>[2x]HGSPVDICTAKPRDIPMNPMCIYRSPEKKATEDEGS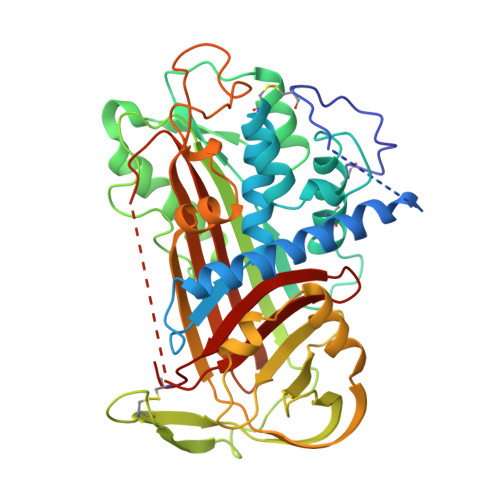EQKIPEATNRRVWELSKANSRFATTFYQHLADSKNDNDNIFLSPLSISTAFAMTKLGACNDTLQQLMEVFKFDTISEKTSDQIHFFFAKLNCRLYRKANKSSKLVSANRLFGDKSLTFNETYQDISELVYGAKLQPLDFKENAEQSRAAINKWVSNKTEGRITDVIPSEAINELTVLVLVNTIYFKGLWKSKFSPENTRKELFYKADGESCSASMMYQEGKFRYRRVAEGTQVLELPFKGDDITMVLILPKPEKSLAKVEKELTPEVLQEWLDELEEMMLVVHMPRFRIEDGFSLKEQLQDMGLVDLFSPEKSKLPGIVAEGRDDLYVSDAFHKAFLEVNEEGSEAAASTAVVIAGRSLNPNRVTFKANRPFLVFIREVPLNTIIFMGRVANPCVK;> SEAAASTAVVIA>[4x]VKVDLESKRYGEKLKEVFLMLDNNVVECIKEITESSRNGKLVFFVGAGVSTLSDYPQWWRLVDKYHEELYGSPKKGNYSSDEYLRIPQIFYNVKGEMAFDGILKDFFQVDKPTNPIHDKILAMNPAHVITTNYDNLIDTACWKRGKYFSVISAEEDVANATSSRYLLKVAGDFRKGFKGENVVLKEDDYLNYDQNYPLISNLMKTIIATHTIVFIGYGLGDYNINMLLNWVRKLQKDSFHKPFFIRTDPSPIENETLIYYENKGLRIIDAASLIDSNEYDYLERYSAVMDLLIESQENKFITKDDEVIDYIYGKISPLFALQYIRKIDLKHVFEYDYHFEVNGTVVRHKNKGFGYMERFFELKESCDERSKLSKKQYERFNALFNFFEKNGVICMAKDAGTLNTSIEINSLAYHGKYDVMKKFIEEQSVSIEDDYKKAFFLACLGRWEESYDLYSNIILNSIDESNGCVYYLSQINRYRIYQSITQAVTQFNGLGLLTFGRHYKPFTDEFLARIEREMTNFNIDD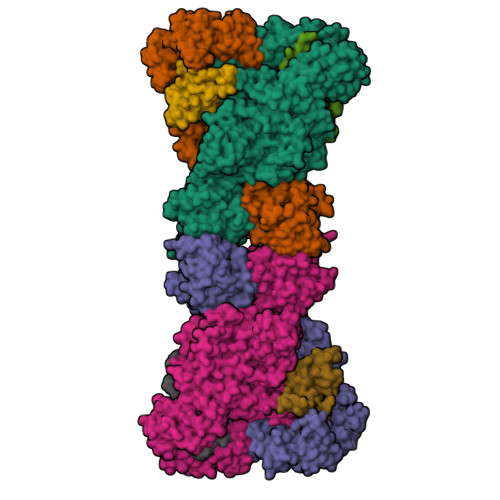LFNGMPFEFQKKYKILEFLSDNQFLYDDTVKLFELTNKVRSEMSEGSYSFGMSSDIVVLLRLYDNLRFLYENCLWSVSFHEFHQYIRNSMSLLIEKAEYERTRDIDELGFSFFGKKSGFFMEYYDFVNISRHFKIDDIKNLERSCSIDKIRFGEQEKIEEYLVGIAEEITKQFSANGMNVVFYTQFISEAKAALYFAKYVKLSEEGLGKIVKALLFYFPERDLDIGKRYVWLERLTKCNELPKSIISIIDDFLVLQAEKHIDQNYSEVSSNGLYSRDYGALIKHFEKNFISKRLSEITLCLTQDKQKQIDFLFKLLPLLSTNAKSHLLSFKSVENINDLMNGIRIGLIDEFTPEHEELIIEYLETRKVNYIVEKEKGIQTFSSNDYMSTFGIWYFLEEINNSKMEEFIGMDDQYDFFVDPENFDYKKFIPSWLKNYNDKLLGKIAGNKHMKHHVIEVLKERVKNSNDKRYLEILMNYFI;>MKTVIQDTADVYFKRKSDGKLVFTAEAQTASFSQAISEEKLRGGIGNKPLYILKSEKEINLTVKNAFFDLEWLAMTQGETIQEETKVKVFDREHGLIVDDTNKVTLKGKPVSDVTFYNKKGLTYKIAVSTDGTYTIPTAFAAAKDKLTAVYQIEKVGRRLAIKASKFSERYEVEYRTIAYNPDTEEVYSDIYIQFPNVSPSGEFEMSLENGNALAPEIKFEALADTDTDEMAVVIEASRDENTAAPVEDTTGSTQSSDLGGTTE[4x]> MMIRGIRGATTVERDTEEEILQKTKQLLEKIIEENHTKPEDVVQMLLSATPDLHAVFPAKAVRELSGWQYVPVTCMQEMDVTGGLKKKISVMMTVQTDVPQDQIRHVYLEKAVVLRPDLSLT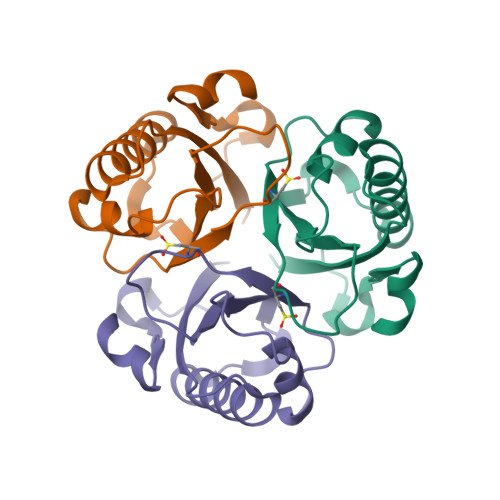KNTEL3-amino-N-ethyl-N-methylbenzamide | C10 H14 N2 O | 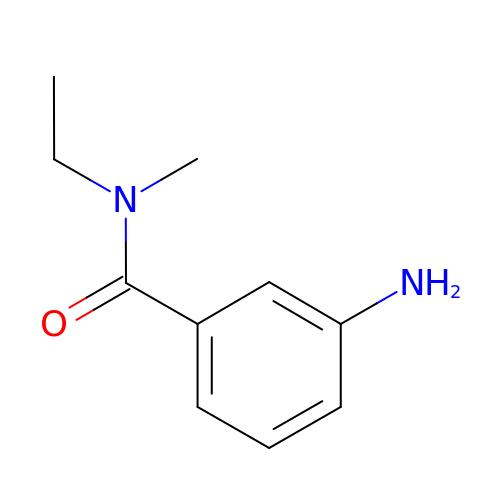URNKFNQWYLXELN-UHFFFAOYSA-N>[2x]MTERIRNVALRSKVCPAETASELIKHGDVVGTSGFTGAGYPKEVPKALAQRMEAAHDRGEKYQISLITGASTGPQLDGELAKANGVYFRSPFNTDATMRNRINAGETEYFDNHLGQVAGRAVQGNYGKFNIALVEATAITEDGGIVPTSSVGNSQTFLNLAEKVIIEVNEWQNPMLEGIHDIWDGNVSGVPTRDIVPIVRADQRVGGPVLRVNPDKIAAIVRTNDRDRNAPFAAPDETAKAIAGYLLDFFGHEVKQNRLPPSLLPLQSGVGNVANAVLEGLKEGPFENLVGYSEVIQDGMLAMLDSGRMRIASASSFSLSPEAAEEINNRMDFFRSKIILRQQDVSNSPGIIRRLGCIAMNGMIEADIYGNVNSTRVMGSKMMNGIGGSGDF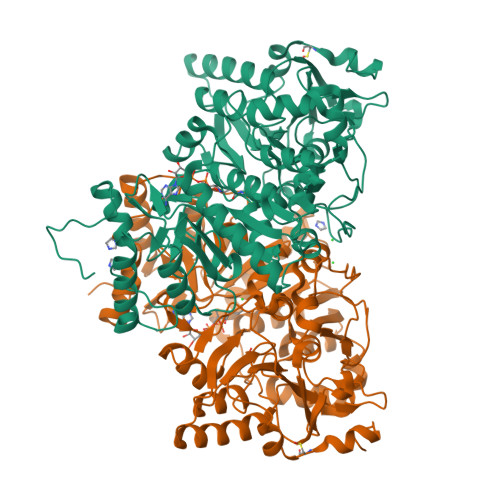ARSSYLSIFLSPSTAKGGKISAIVPMAAHVDHIMQDAQIFVTEQGLADLRGLSPVQRAREIISKCAHPDYRPMLQDYFDRALKNSFGKHTPHLLTEALSWHQRFIDTGTMLPSSLEHHHHHH>MTKQHAFTREDLLRCSRGELFGPGNAQLPAPNMLMIDRIVHISDVGGKYGKGELVAELDINPDLWFFACHFEGDPVMPGCLGLDAMWQLVGFYLGWQGNPGRGRALGSGEVKFFGQVLPTAKKVTYNIHIKRTINR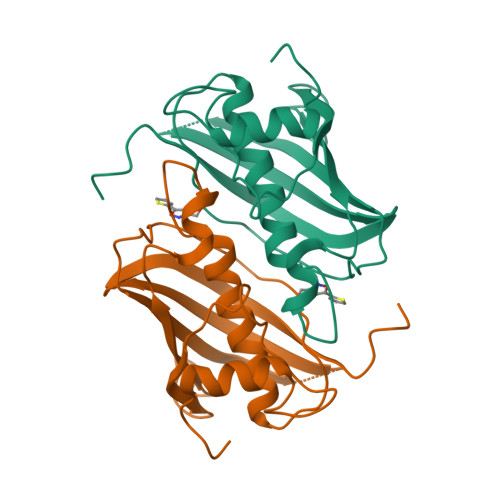SLVLAIADGTVSVDGREIYSAEGLRVGLFTSTDSF[20x]> MGDTKEQRILRYVQQHAKPGDPQSVLEAIDTYCTQKEWAMNVGDAKGQIMDEVIQEHNPSLVLELGAYCGYSAVRMARLLSPGARLLTMEKNPDYAAITQQMLNFAGLQDKVTI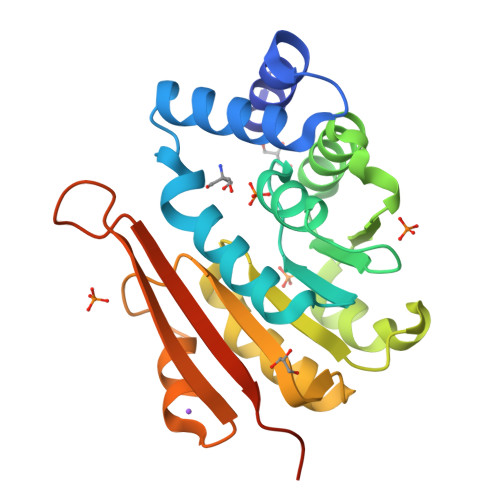LIGASQDLIPQLKKYDVDTLDLVFLDHWKDRYLPDTILLEECGLLRKGTVLLADNVIVPGTPDFLAYVRGSSSFECTHYSSYLEYMKVVDGLEKAVYKGPSSPKQPLEHHHHHH7-[cis-3-(azetidin-1-ylmethyl)cyclobutyl]-5-[3-(benzyloxy)phenyl]-7H-pyrrolo[2,3-d]pyrimidin-4-amine 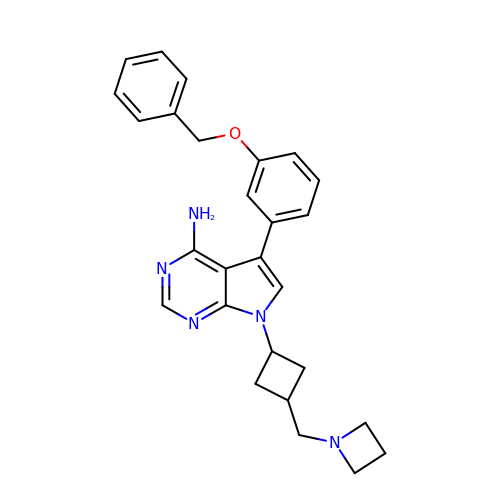| C27 H29 N5 O | AECDBHGVIIRMOI-GRGXKFILSA-N>[2x]MKNFSIAKSRRLRSTPYTSRIEKQGVTAYTIYNHMLLPAAFGSIEDSYKHLKEHV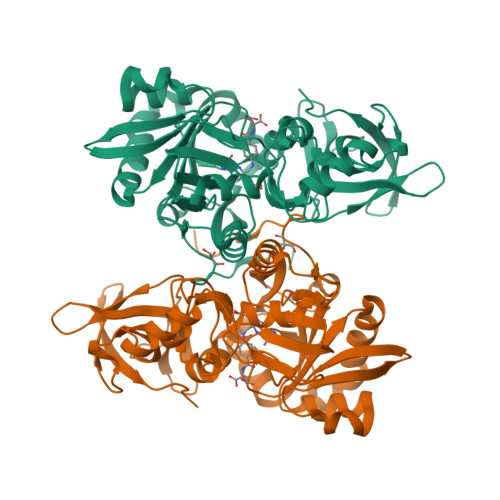QIWDVAAERQVEISGKDSAELVQLMTCRDLSKSKIGRCYYCPIIDENGNLVNDPVVLKLDENKWWISIADSDVIFFAKGLASGHKFDVKIVEPVVDIMAIQGPKSFALMEKVFGKKITELKFFGFDYFDFEGTKHLIARSGWSKQGGYEVYVENTQSGQKLYDHLFEVGKEFNVGPGCPNLIERIESALLSYGNDFDNNDNPFECGFDQYVSLDSDINFLGKEKLKEIKLKGPQKKLRGVKIDIKEISLTGSKNIYDENNNVIGELRSACYSPHFQKVIGIAMIKKSHWEASQGFKIQINDNTINGNVCDLPFI>[2x]AVTTRQITVPSAPMGWASWNSFAAKIDYSVIKKQVDAFVAAGLPAAGYTYINIDEGWWQGTRDSAGNITVDTAEWPGGMSAITAYIHSKGLKAGIYTDAGKDGCGYYYPTGRPAAPGSGSEGHYDQDMLQFSTWGFDFVKVDWCGGDAEGLDAATTYKSISDAVGRAAATTGRPLTLSICNWGYQNPWNWAAGQAPLWRTSTDIIYYGNQPSMTSLLSNFDQTLHPTAQHTGYYNDPDMLMVGMDGFTAAQNRTHMNLWAISGAPLLAGNDLTTMTSETAGILKNPEVIAVDQDSRGLQGVKVAEDTTGLQAYGKVLSGTGNRAVVLLNRTSAAHDITVRWSDLGLTNASATVRDLWARQNVGTSATGYTASVPAGGSVMLT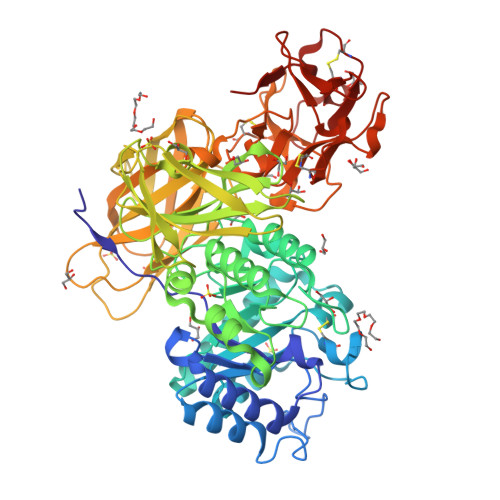VTGGTEAAGGAYAATSTGRYTGVTAASTGLNVVDVAYTNNTSSARTATLQVNGQTATTVSFPPTGASAGTVSVEVSLSKGSANTLALSGGPATEGITVRPLPGTNGALVTGKQSGRCADIYNNTITNGTQAELWDCNGGPNQSWTYTSRKELVLYGNKCLDAYNLGTTNGTKVVIWDCNGQANQKWNINSDGTITNVNAGLCLDAYNAATANGTSLVLWSCGTGDNQKWTVT> LIEVKNLSFNRGERVIYDNISLNIRRGQITAIMGPSGTGKTTLLRLIGGQLVPDQGEVLLDGKDIAQMSRQRARMGMLFQSGALFTDMSVYENVAFP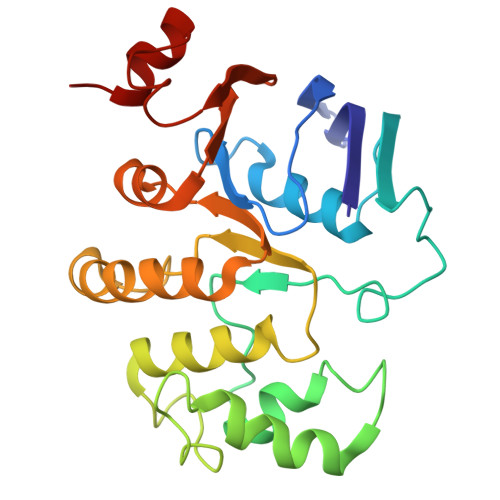IRAHTLSENLIAELVALKLESVGLRGTEQLMPTELSGGMNRRVALARAIALDPDLIMYDEPFAGQDPIVKGVLTRLIRSLREALDLTTIIVSHDVPETLSIADYIYVVAEGKIQGEGTPEELQAYASPFVKQFLTG>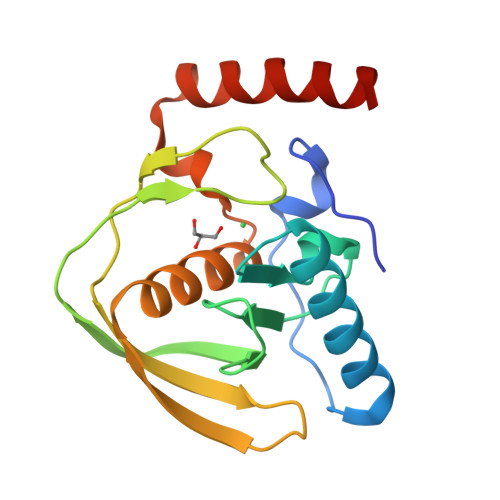[4x]MTALNVLIYPDDHLKVVCEPVTEVNDAIRKIVDDMFDTMYQEKGIGLAAPQVDILQRIITIDVEGDKQNQFVLINPEILASEGETGIEEGCLSIPGFRALVPRKEKVTVRALDRDGKEFTLDADGLLAICIQHEIDHLNGILFVDYLSPLKRQRIKEKLIKYKKQIAKS>[2x]MAKKTSSKGKEGVGSSSVSFPCLPRLPLLGSLLHLRSNLPPHLLFTQLSSQYGPLFGLYAGPHLTLVVSEIGLVREVLLQRGREFAGRPKMVTTDLLTQGGKDIAFADYSPLWKNHRRLVHSSFTLFGEGS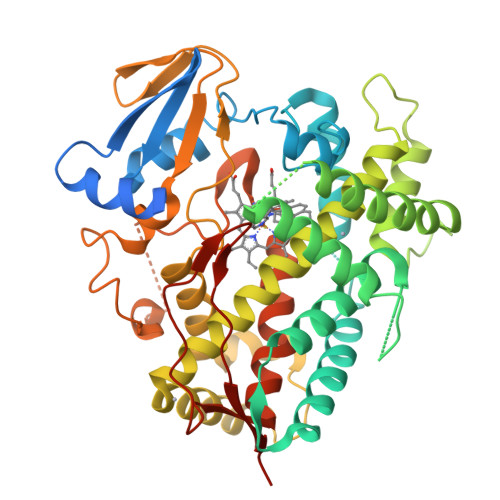NKLQTIVQEAADSLCEELQACRGQSSDLSVVLMRAVTNVICRLVFSSSYQPSDPELQTVIQYNDGIVQTIARGGLVDIFPWLRIFPNKDLKRLKECVSIRDQLLYKKLLEHKKSLTPGEPRDLLDALLIGQQRGSGGADDITEDHVLMTAAEAFGAGVETTSTTLLWTIAFLLHHPQLQERVQAELDECVGVDRPPCLSDRPHLPLLDAVLCEVMRIRPVSPILIPHVAMQDTSLGGHSVPKGTRVLVNMWAIHHDPKHWDQPEQFNPERFLEPSGKKKTQSSFLPFGAGPRVCVGESLARIELFLFVSRPLQRFSFSCPSEASLPDLQGRFGVVLQPERYTVTVTPRHHHHHHH>WSADNPTNTDVNTHYWLFKQAEKILAKDVNHMRANLMNELKKFDKQIAQGIYDADHKNPYYDTSTFLSHFYNPDRDNTYLPGFANAKITGAKYFNQSVTDYREGKFDTAFYKLGLAIHYYTDISQPMHANNFTAISYPPGYHSAYENYVDTIKHNYQATEDMVAKRFSSDDVKDWLYENAKRAKADYPKIVNAKTKKSYLVGNSEWKKDTVEPTGARLRDSQQTLAGFLEFWSKKTNE[2x]

Listeriosis is one of the most serious foodborne diseases caused by the intracellular bacterium Listeria monocytogenes. Its two major virulence factors, broad-range phospholipase C (LmPC-PLC) and the pore-forming toxin listeriolysin O (LLO), enable the bacterium to spread in the host by destroying cell membranes. Two phospholipases C (PLCs), phosphatidyl inositol specific (LmPI-PLC or PlcA) and broad-range (LmPC-PLC or PlcB), facilitate vacuolar escape of Lm by cooperating with LLO in vacuolar membrane disruption. Homologs of LmPC-PLC, which belong to the family of Zn2+-dependent phospholipases, have so far only been found in the genera Bacillus and Clostridium. LmPC-PLC exhibits broad substrate specificity, with the highest activities towards glycerophospholipids with phosphocholine, phosphoserine, and phosphoethanolamine head groups, but less towards phosphoglycerol or phosphoinositol head groups, and also hydrolyses sphingomyelin (SM).

Of all the constructs, LmPC-PLCC143S+C168S had the highest solubility and successfully produced crystals. Therefore, to determine the crystal structure of LmPC-PLCC143S+C168S (referred to as the crystal structure of LmPC-PLC in the rest of the text), we used X-rays with a wavelength of 1.26 Å near the absorption edge of Zn, based on previous studies suggesting that three Zn ions are in the active site of LmPC-PLC26 and the Bc and Cp homologs. LmPC-PLC crystallized in space group P212121 with two molecules, molA and molB, in the asymmetric unit, whose structures were determined at 2 Å resolution. Three metal ions were found bound to the active site in molA, and only two in molB. Interestingly, while the strength of the anomalous signal at the metal ion position 3 was comparable between the anomalous difference maps of 1.26 Å and 1.33 Å data, the anomalous signal at metal ion position 2 was significantly weaker in the anomalous difference map of the data collected at 1.33 Å, suggesting that the metal ion position 2 may contain Fe ions in some molecules and Zn ions in others. The absence of a pronounced electron density in the anomalous difference map in molB at metal position 1 and the shorter distance between H69 and H118 than in molA indicated that no Zn or other metal ion was present at this position in molB. A glycerol molecule was bound in the active site of both molecules, originating from either the bacterial growth medium or the cell lysis buffer. Interestingly, the N-terminal residue W1 is well defined by electron density in both LmPC-PLC structures, while there was no traceable density for the following residues S2 to T9 connecting W1 to the αA-helix. LmPC-PLC molB, with its partially occluded active site by the D55-S64 loop and the absence of Zn1, could represent the closed, inactive state, and molA with a more open active site due to the flexibility of the D55-S64 loop and Zn ion in place, could represent the open, active state.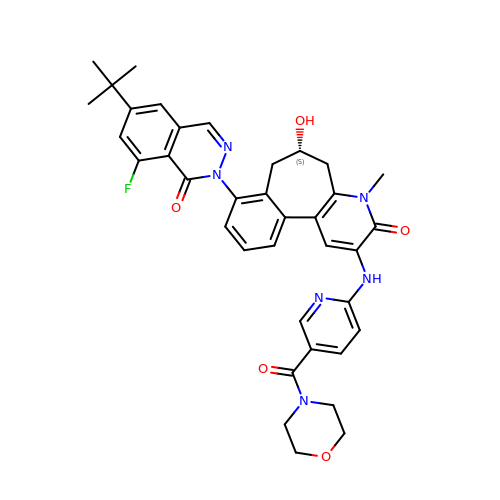(9~{S})-12-(6-~{tert}-butyl-8-fluoranyl-1-oxidanylidene-phthalazin-2-yl)-6-methyl-4-[(5-morpholin-4-ylcarbonylpyridin-2-yl)amino]-9-oxidanyl-6-azatricyclo[9.4.0.0^{2,7}]pentadeca-1(15),2(7),3,11,13-pentaen-5-one | C37 H37 F N6 O5 | ACFBKRAWAGNCMP-DEOSSOPVSA-N[(2~{S})-1-octadecanoyloxy-3-[oxidanyl-[(1~{R},2~{R},3~{S},4~{S},5~{S},6~{S})-2,3,6-tris(oxidanyl)-4,5-diphosphonooxy-cyclohexyl]oxy-phosphoryl]oxy-propan-2-yl] icosa-5,8,11,14-tetraenoate | C47 H85 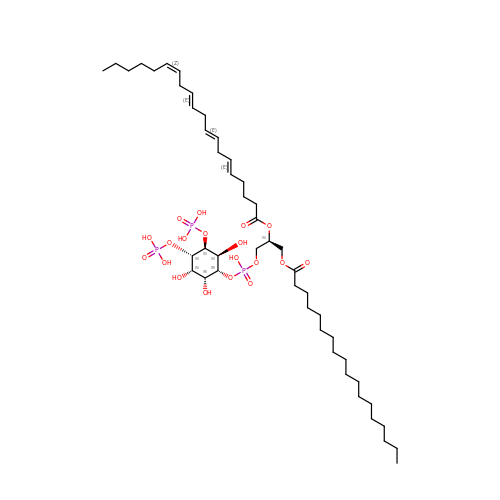O19 P3 | CNWINRVXAYPOMW-UWUKCHIJSA-N CYTIDINE-5'-DIPHOSPHATE | C9 H15 N3 O11 P2 | 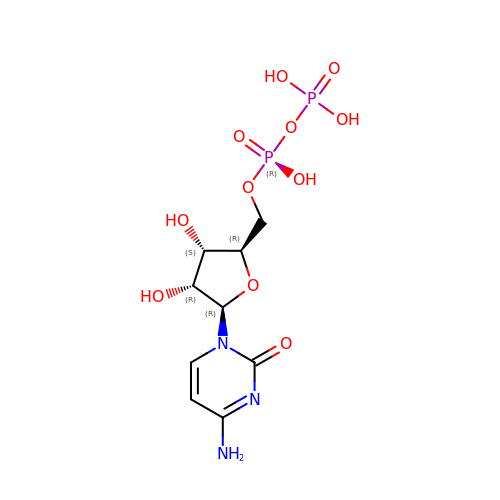ZWIADYZPOWUWEW-XVFCMESISA-N>MMIIDCHGHYTVLPKAHDEWREQQKAAFKAGQPAPPYPEISDDEIRETIEANQLRLIKERGADMTIFSPRASAMAPHVGDQSVAVPWAQACNNLIARVVDLFPETFAGVCMLPQSPEADMTSSIAELERCVNELGFIGCNLNPDPGGGHFKHPPLTDRFWYPFYEKMVELDVPAMIHVSGSCNPAMHATGAYYLAADTIAFMQLLQGNLFADFPTLRFIIPHGGGAVPYHWGRFRGLADMLKQPSLDTLLMNNVFFDTCV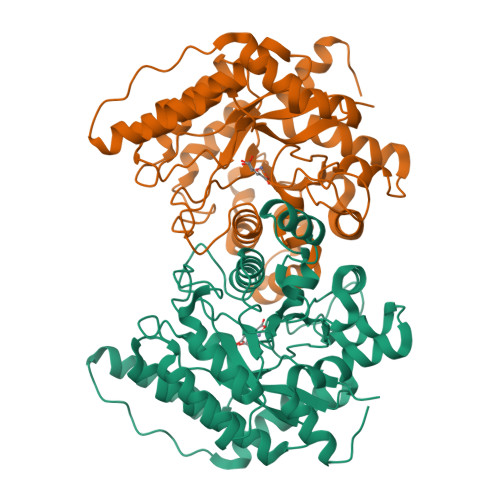YHQPGINLLADVIDNKNILFGSQMVGAVRGIDPTTGHYFDDTKRYIDALDISDQERHAIFEGNTRRVFPRLDAKLKARGLLE[4x]>GPGSMAKNQWRPYTNGSHAPSTPRHLLSIADLTPTEFATLVRNASSYKKTIKSDSMPERLTGALSGKTVAMMFSKRSTRTRVSTEGAVVKMGGHPMFLGKDDIQLGVNESLYDTSVVISSMVSCIVARVGPHSDIANLAKHSSVPVINALCDTFHPLQAIADFLTIHESFASQSATHGTHPSSLGLEGLKIAWVGDANNVLFDLAIAATKMGVNVAVATPRGYEIPSHIVELIQKAREGVQSPGNLTQTTVPEVAVKDADVIVTDTWISMGQETEKIKRLEAFK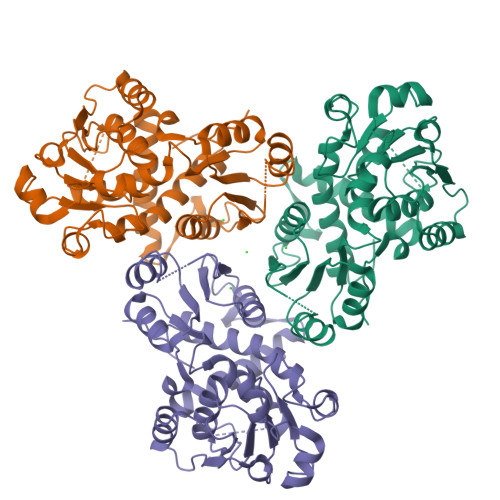DFKVTSELAKRGGAKENWKFMHCLPRHPEEVSDEVFYSERSLVFPEAENRLWAAISALEAFVVNKGKIA[3x]> TWGVSSPKNVQGLSGSCLLIPCIFSYPADVPVSNGITAIWYYDYSGKRQVVIHSGDPKLVDKRFRGRAEL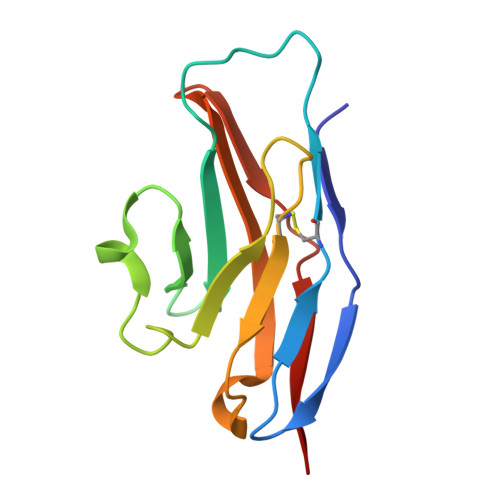MGNMDHKVCNLLLKDLKPEDSGTYNFRFEISDSNRWLDVKGTTVTVTT> GSHMSEKEIRRSMPLFPIGPVMKLTDLTARQIRYYEDQGLIHPARNQGNHRLYSLQDIDVLLEIKDYLNDGLNIAGIKKMYQMQQKESKEPLTDDDVRKILRKEMQQAGRFVKQDATGKQQLPRF

In Gram-positive bacteria, nitrogen homeostasis is controlled by an operon encoding glutamine synthetase (GS), a dodecameric machine that assimilates ammonium into glutamine, and the GlnR repressor. GlnR detects nitrogen excess indirectly by binding glutamine-feedback-inhibited-GS (FBI-GS), which activates its transcription-repression function. GS generates glutamine from glutamate, ATP, and ammonium by a mechanism that involves the initial phosphorylation of the γ-carboxyl group of glutamate by ATP and the subsequent incorporation of ammonium. The structures show FBI-GS binds the GlnR C-terminal domain within its active-site cavity, juxtaposing two GlnR monomers to form a DNA-binding-competent GlnR dimer.

We next obtained structures of Sa GlnR and Lm GlnR bound to a 21 bp glnR consensus operator site to 2.35 and 3.45 Å, respectively, by X-ray crystallography. The GlnR structures are similar to each other and the Bs GlnR (rmsd = 0.6–0.8 Å for overlay of 67 corresponding Cα atoms). Residues 2–73 and 2–83 were visible for the Lm and Sa GlnR proteins respectively. The Lm and Sa GlnRs form comparable dimers to the Bs GlnR and dock on the DNA similarly. As observed in the Bs structure, both DNA sites bound by Sa and Lm GlnR are bent inward but the DNA from the Lm complex is slightly less bent (~21°) compared to the Sa and Bs structures (~25°). The GlnR DNA used for crystallization contains four conserved bps (bolded) in each half-site, 5′-CGTGTCAGATAATCTGACACG-3′ (where the consensus binding site is N1N2T3G4T5N6A7N(7)T7’N6’A5’C4’A3’N2’N1’; N indicates any nucleotide). These conserved bps are contacted in the major groove by Lm and Sa GlnR residues that are completely conserved among GlnRs; a conserved tyrosine (Sa Tyr32/Lm Tyr31) makes hydrophobic contacts to the DNA thymine3 (T3) methyl group, an arginine (Sa Arg28/Lm Arg27) specifically reads the G4 base and makes hydrophobic interactions with the methyl moiety of T5 and finally, the side chain methylene carbons of a conserved arginine (Sa Arg31/Lm Arg30) contacts the T7′ methyl group. However, GlnR proteins contain different wing residues, which our structures show make distinct contacts to the minor groove; wing residues Bs Arg46 and Sa Lys48 make nonspecific base contacts in the minor groove, but the corresponding Lm GlnR residue, His47, makes hydrophobic contacts to a ribose. The lack of minor groove base contacts by Lm GlnR may explain the slightly reduced DNA bend observed in this structure as the minor groove base contacts by Bs Arg46 and Sa Lys48 are facilitated by the more bent DNA conformation. The Sa GlnR dimer is generated by interacting N-terminal loops, while the Lm and the Bs N-terminal regions fold into distorted helices that interact. Nonetheless, all these interfaces bury significantly less surface area (~300–400 Å2 BSA) than the >2000 Å2 shielded by physiologically relevant dimers.Aquaporin-7 (AQP7)—together with AQPs 3, 9, and 10—belongs to the aquaglyceroporin subgroup of the AQP family based on sequence homology and permeability to H2O, glycerol, urea, purines, and arsenite. Moreover, AQP7 is abundantly expressed in human adipose tissue, where during lipolysis it mediates the efflux of newly generated glycerol. Structurally, all AQPs share a tetrameric configuration with each functionally independent monomer composed of six membrane-spanning helices (H1-H6) arranged in a right-handed helical bundle. H1-H6 and two short α-helical segments (HB and HE), provide the framework for the internal monomeric pore with its selectivity filter (SF), built in AQP7 from residues F74, G222, Y223, and R229.

In our AQP7 structure, X-ray crystallography captures AQP7 monomeric pores in a unique closed state in which F74 and Y223 block passage of small solutes. Crystal packing analysis reveals 2 stacked AQP7 tetramers interfaced at the EV so that neither the N- nor C-termini participate in crystal contacts. Despite a resolution of 3.95 Å the high crystal symmetry (F4132) and additional presence of non-crystallographic symmetry (NCS) makes it possible, in symmetry-averaged maps, to resolve electron-density features of many amino-acid side-chains as indicated in Figure 3B. Uniquely in AQP7, the NPA motifs are NPS/NAA, eliminating the proline-stacking interaction characteristic of nearly all AQPs. The crystal structure of AQP7 reveals (a) the arrangement of the NAA (94–96) and NPS motifs that form the NPA constriction in AQP7, where the van der Waals packing of A95 and P227 in AQP7 replaces that of the conserved prolines in GlpF; and (b) that residues F74 and Y223 in the SF establish a wedge that excludes glycerol, suggesting that our structure captures a closed state. The SF of AQP7 can exist in two alternate states, one represented by our structure, with constriction diameters of only 2.1 Å or 2.2 Å in each monomer, and an alternate state revealed by MD simulations, with a constriction diameter of 3.5 Å. Although H2O would permeate through the narrow SF constriction in our AQP7 structure, the hydrophobic wedge formed by F74 and Y223 in AQP7 cannot accommodate the larger glycerol molecule. Moreover, 2Fo-Fc simulated annealing omit maps show clear average densities consistent with glycerol in all 4 monomeric pores of AQP7. The two NCS-related AQP7 dimers comprise two monomers with 3 glycerol molecules (Glycerols), and two monomers with 2 glycerol molecules in the monomeric pore. Interestingly, monomers with the inward-facing Y67 orientation house only two glycerol molecules, whereas monomers with the outward-facing orientation of Y67 have three glycerols. In stark contrast to GlpF, we observe no ligand electron density at the selectivity filter of AQP7 (SF).

>[4x]MVQASGHRRSTRGSKMVSWSVIAKIQEILQRKMVREFLAEFMSTYVMMVFGLGSVAHMVLNKKYGSYLGVNLGFGFGVTMGVHVAGRISGAHMNAAVTFANCALGRVPWRKFPVYVLGQFLGSFLAAATIYSLFYTAILHFSGGQLMVTGPVATAGIFATYLPDHMTLWRGFLNEAWLTGMLQLCLFAITDQENNPALPGTEALVIGILVVIIGVSLGMNTGYAINPSRDLPPRIFTFIAGWGKQVFSNGENWWWVPVVAPLLGAYLGGIIYLVFIGSTIPREPLKLEDSVAYEDHGITVLPKMGSHEPTISPLTPVSVSPANRSSVHPAPPLHESMALEHFGGSLEVLFQGPAAYPYDVPDYAAAHHHHHHHHHH> MSIKDEIYNIFNADGKILQIEYGLEAVNKSLPLVVLKNKNMIVCAAKKNQGHLLEDEVQTSFQPIYPNLYSAFTGNWADVFYVNSKAKDLAHYASYKLGFSVTPDILCRKLADELQPLIQSTGERAPAFAGALFGFDNGKPVVYMTNISAVCYPVYG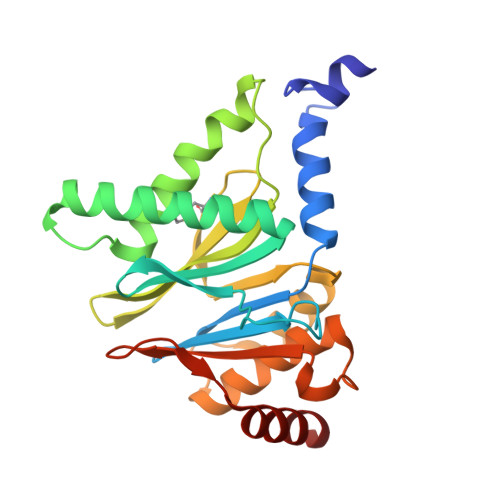SMVGSKNQNMYKYVEKYYNEDIEDEKLFEVAVGGLLESLGENSVYQEMEVAYLRNGEVLKYLDDKEIESLLLSIADK> MAHHHHHHDDDDKGSMS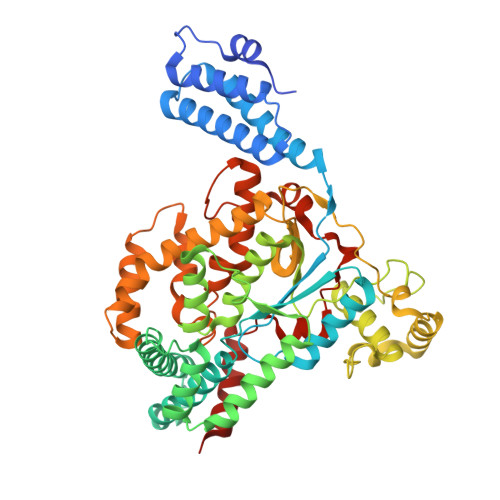LISKEELIKLAYSIRPRENEYKTILTNLDEYNKLTTNNNENKYLQLKKLNESIDVFMNKYKTSSRNRALSNLKKDILKEVILIKNSNTSPVEKNLHFVWIGGEVSDIALEYIKQWADINAEYNIKLWYDSEAFLVNTLKKAIVESSTTEALQLLEEEIQNPQFDNMKFYKKRMEFIYDRQKRFINYYKSQINKPTVPTIDDIIKSHLVSEYNRDETVLESYRTNSLRKINSNHGIDIRANSLFTEQELLNIYSQELLNRGNLAAASDIVRLLALKNFGGVYLDVDMLPGIHSDLFKTISRPSSIGLDRWEMIKLEAIMKYKKYINNYTSENFDKLDQQLKDNFKLIIESKSEKSEIFSKLENLNVSDLEIKIAFALGSVINQALISKQGSYLTNLVIEQVKNRYQFLNQHLNPAIESDNNFTDTTKIFHDSLFNSATAENSMFLTKIAPYLQVGFMPEARSTISLSGPGAYASAYYDFINLQENTIEKTLKASDLIEFKFPENNLSQLTEQEINSLWSFDQASAKYQFEKYVRDYTGGS> GAVSIEPRINVGSRFQAEIPLMRDRALAAADPHKADLV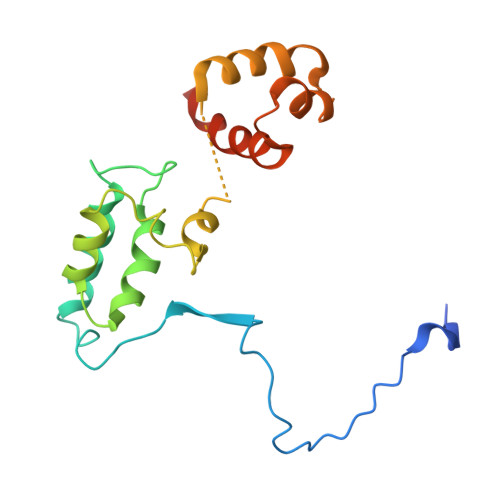WQPWEDLESSREKQRQVEDLLTAACSSIFPGAGTNQELALHCLHESRGDILETLNKLLLKKPLRPHNHPLATYHYTGSDQWKMAERKLFNKGIAIYKKDFFLVQKLIQTKTVAQCVEFYYTYKKQVKIGRNGTLT> HHHHHHNRPRFTLQELRDVLQERNKLKSQL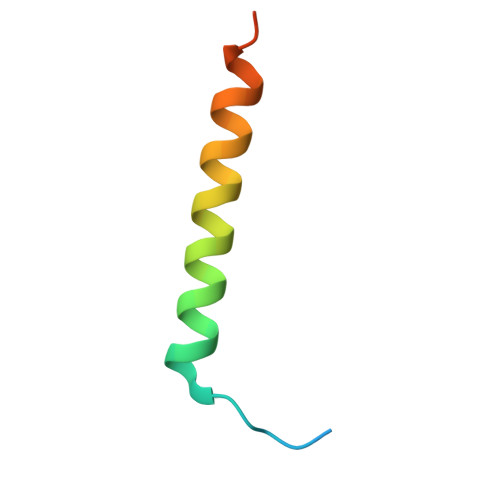LVVQEELQCYKSG> MGSSHHHHHHSSGENLYFQGSHMTATATSAK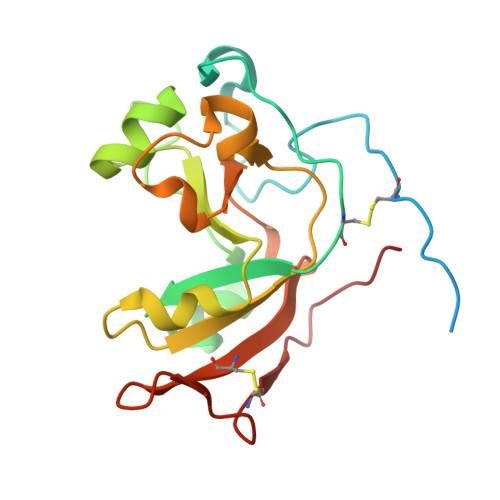AAAPACPRFDDPVHAAADPRVDVERITPDPVWRTTCGTLYRSDSRGPAVVFEQGFLPKDVIDGQYDIESYVLVNQPSPYVSTTYDHDLYKTWHKSGYNYYIDAPGGVDVNKTIGDRHKWADQVEVAFPGGIRTEFVIGVCPVDKKTRTEKMSECVGNPHYEPWH>TKEERVLLMKVAILAIVAAKKGNTDEVRKALELALLIAKVSGTTEAVKLALEVVARVAIEAARRGNTDAVREALEVALEIARESGTTEAVKLALEVVARVAIEAARRGNTEAVVEALLVALEIAKESGTEEAVRLALEVVKRVSNEALK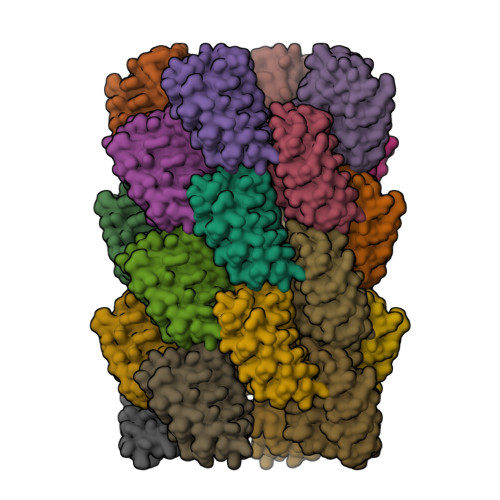QGNVDAVKVALEVRKMIEELSG[24x]>MSEMSSFLHIGDIVSLYAEGSVNGFISTLGLVDDRCVVEPAAGDLDNPPKKFRDCLFKVCPMNRYSAQKQYWKAKQTKQDKEKIADVVLLQKLQHAAQMEQKQNDTENKKVHGDVVKYGSVIQLLHMKSNKYLTVNKRLPALLEKNAMRVTLDATGNEGSWLFIQPFWKLRSNGDNVVVGDKVILNPVNAGQPLHASNYELSDNAGCKEVNSVNCNTSWKINLFMQFRDHLEEVLKGGDVVRLFHAEQEKFLTCDEYKGKLQVFLRTTLRQSATSATSSNALWEVEVVHHDPCRGGAGHWNGLYRFKHLATGNYLAAEENPSYKGDASDPKAAGMGAQGRTGRRNAGEKIKYCLVAVPHGNDIASLFELDPTTLQKTDSFVPRNSYVRLRHLCTNTWIQSTNVPIDIEEERPIRLMLGTCPTKEDKEAFAIVSVPVSEIRDLDFANDASSMLASAVEKLNEGFISQNDRRFVIQLLEDLVFFVSDVPNNGQNVLDIMVTKPNRERQKLMREQNILKQVFGILKAPFREKGGEGPLVRLEELSDQKNAPYQHMFRLCYRVLRHSQEDYRKNQEHIAKQFGMMQSQIGYDILAEDTITALLHNNRKLLEKHITKTEVETFVSLVRKNREPRFLDYLSDLCVSNHIAIPVTQELICKCVLDPKNSDILIRTELRPVKEMAQSHEYLSIEYSEEEVWLTWTDKNNEHHEKSVRQLAQEARAGNAHDENVLSYYRYQLKLFARMCLDRQYLAIDEISQQLGVDLIFLCMADEMLPFDLRASFCHLMLHVHVDRDPQELVTPVKFARLWTEIPTAITIKDYDSNLNASRDDKKNKFANTMEFVEDYLNNVVSEAVPFANEEKNKLTFEVVSLAHNLIYFGFYSFSELLRLTRTLLGIIDCVQGPPAMLQAYEDPGGKNVRRSIQGVGHMMSTMVLSRKQSVFSAPSLSAGASAAEPLDRSKFEENEDIVVMETKLKILEILQFILNVRLDYRISYLLSVFKKEFVEVFPMQDSGADGTAPAFDSTTANMNLDRIGEQAEAMFGVGKTSSMLEVDDEGGRMFLRVLIHLTMHDYAPLVSGALQLLFKHFSQRQEAMHTFKQVQLLISAQDVENYKVIKSELDRLRTMVEKSELWVDKKGSGKGEEVEAGAAKDKKERPTDEEGFLHPPGEKSSENYQIVKGILERLNKMCGVGEQMRKKQQRLLKNMDAHKVMLDLLQIPYDKGDAKMMEILRYTHQFLQKFCAGNPGNQALLHKHLHLFLTPGLLEAETMQHIFLNNYQLCSEISEPVLQHFVHLLATHGRHVQYLDFLHTVIKAEGKYVKKCQDMIMTELTNAGDDVVVFYNDKASLAHLLDMMKAARDGVEDHSPLMYHISLVDLLAACAEGKNVYTEIKCTSLLPLEDVVSVVTHEDCITEVKMAYVNFVNHCYVDTEVEMKEIYTSNHIWTLFENFTLDMARVCSKREKRVADPTLEKYVLSVVLDTINAFFSSPFSENSTSLQTHQTIVVQLLQSTTRLLECPWLQQQHKGSVEACIRTLAMVAKGRAILLPMDLDAHISSMLSSGASCAAAAQRNASSYKATTRAFPRVTPTANQWDYKNIIEKLQDIITALEERLKPLVQAELSVLVDVLHWPELLFLEGSEAYQRCESGGFLSKLIQHTKDLMESEEKLCIKVLRTLQQMLLKKTKYGDRGNQLRKMLLQNYLQNRKSTSRGDLPDPIGTGLDPDWSAIAATQCRLDKEGATKLVCDLITSTKNEKIFQESIGLAIHLLDGGNTEIQKSFHNLMMSDKKSERFFKVLHDRMKRAQQETKSTVAVNMNDLGSQPHEDREPVDPTTKGRVASFSIPGSSSRYSLGPSLRRGHEVSERVQSSEMGTSVLIMQPILRFLQLLCENHNRDLQNFLRCQNNKTNYNLVCETLQFLDIMCGSTTGGLGLLGLYINEDNVGLVIQTLETLTEYCQGPCHENQTCIVTHESNGIDIITALILNDISPLCKYRMDLVLQLKDNASKLLLALMESRHDSENAERILISLRPQELVDVIKKAYLQEEERENSEVSPREVGHNIYILALQLSRHNKQLQHLLKPVKRIQEEEAEGISSMLSLNNKQLSQMLKSSAPAQEEEEDPLAYYENHTSQIEIVRQDRSMEQIVFPVPGICQFLTEETKHRLFTTTEQDEQGSKVSDFFDQSSFLHNEMEWQRKLRSMPLIYWFSRRMTLWGSISFNLAVFINIIIAFFYPYMEGASTGVLDSPLISLLFWILICFSIAALFTKRYSIRPLIVALILRSIYYLGIGPTLNILGALNLTNKIVFVVSFVGNRGTFIRGYKAMVMDMEFLYHVGYILTSVLGLFAHELFYSILLFDLIYREETLFNVIKSVTRNGRSILLTALLALILVYLFSIVGFLFLKDDFILEVDRLPNNHSTASPLGMPHGAAAFVDTCSGDKMDCVSGLSVPEVLEEDRELDSTERACDTLLMCIVTVMNHGLRNGGGVGDILRKPSKDESLFPARVVYDLLFFFIVIIIVLNLIFGVIIDTFADLRSEKQKKEEILKTTCFICGLERDKFDNKTVSFEEHIKLEHNMWNYLYFIVLVRVKNKTDYTGPESYVAQMIKNKNLDWFPRMRAMSLVSNEGEGEQNEIRILQDKLNSTMKLVSHLTAQLNELKEQMTEQRKRRQRLGFVDVQNCISR[4x]

Inositol-1,4,5-trisphosphate receptors (IP3Rs) are large, tetrameric cation channels that serve as the primary intracellular calcium (Ca2+) release channels in nonexcitable cells. Expressed in the endoplasmic reticulum (ER), IP3Rs mediate the flow of Ca2+ from the ER into the cytoplasm and other cellular compartments where Ca2+ contributes to the regulation of cell division, differentiation, metabolism, migration, and cell death. Notably, IP3Rs are inhibited by micromolar cytosolic Ca2+ concentrations, resulting in a biphasic dependence on Ca2+ for channel activity. Here, we collect electron cryomicroscopic images of human type 3 IP3R (hIP3R3) vitrified in a broad range of Ca2+ concentrations and treat particle abundance as a proxy for the relative free energy of each state to establish high-resolution thermodynamic models of IP3R activation and inhibition, which combined with cellular Ca2+ imaging elucidates the structural basis for IP3R-generated Ca2+ oscillations.

In the first of the major states, the BTF ring is intact, ARM2 is extended, the JD ring is intact, and the pore is closed. In both the resting and preactivated states, no density peaks consistent with a bound Ca2+ ion were observed at either the JD or CD binding sites. The IP3-binding site is best resolved in the resting state where Arg568 on ARM1 coordinates the 1-phosphate of IP3 conferring a specific orientation to IP3 in this pocket as predicted by mutagenesis. For example, the abundance of the putative resting state, which closely resembles the ligand-free state and shows no evidence of bound Ca2+ ions, is negatively correlated with the concentration of Ca2+. At low Ca2+, 45.2% of the particles adopt the resting state whereas this percentage drops to 0.7% at high Ca2+. In the resting state, a portion of the wedge loop, including Thr926-Ala943, inserts into a cavity surrounded by the CLD, ARM1, ARM2 and ARM3 and adopts an ordered conformation. By aligning the maps based on the strength of the density for the wedge loop, we found that the flexibility of ARM2, as assessed by the local quality of the density, is inversely correlated with the strength of the wedge loop density, indicating that the presence of the wedge loop stabilizes ARM2 in the extended conformation. IP3 generated in response to extracellular stimuli can bind to the ligand-free channel without altering its global conformation, yielding the low-energy resting state. At low Ca2+ IP3Rs must escape a low-energy ARM2 extended resting state in order to activate by binding Ca2+ at the high-affinity JD site.> SNRTSAKSNLMLILLGLQMKEISNSDLYKLKEVRSVVTSLASFLFQQQNVGVMKSFDSL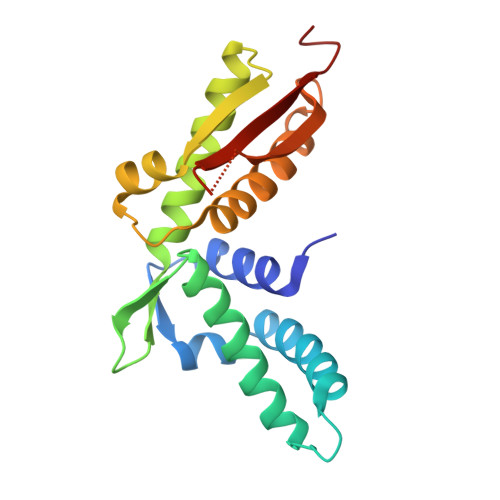EKEAFRDLVNRLVSQGLIGLKDKTSETFDLLPLKNLFEYAEKRISVLMKLQCYTGTVQLSHVQEKLHLPYITTNGIVDVFKECLKRTKKQYPEVLKNWWIDLDPKNGMEDQNSGILLHLEYAAAYS>MAGLSVSDHLDGQLARLCEVAGADPVEPRNLLAGLLGPVGPRPLYEPPAWPSGVSDDHTPVEFSIAFNEAEPPTLRILGETLGSPPGPLANLSATRGFLDAQARRAGLSTSRLDSVRDLFATDDPQGDFAMWCSLVFRSSRRPEFKVYLNPEVKGVERS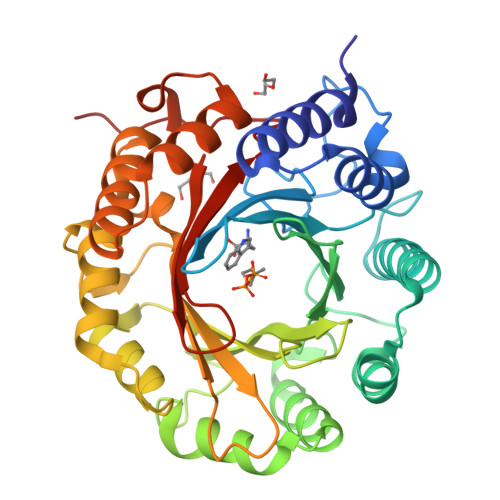PALVSEALHRLGLGASYRALLDHGVRPGELGRGDRLTFFAVDLHDGPQARVKLYLTHHEAEVWDVTRAASVVDGVDVAEIEEFCVVAGGGTRRFDGRPLVGSYTFTEGADRPVGYSIYVPIRSYVTDDQEARDRVAALLVRYGFDTDGLDRAIAAVTPRPLRDGVGLIAHVSLRLGAPRPGVTVYLSAEAYRVSPPRPRLVPR[4x]6-(3-amino-2H-indazol-6-yl)-N~4~-ethylpyrimidine-2,4-diamine 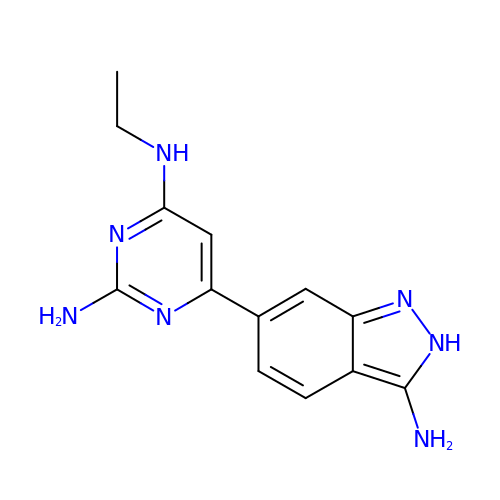| C13 H15 N7 | RIXHCYHQTKRWDU-UHFFFAOYSA-N>[2x]MNIQSTIKAVAETISTGPIPGSRKVYQAGELFPELRVPFREVAVHPSANEPPVTIYDPSGPYSDPAIQIDIEKGLPRTREALVVARGDVEEVADPRQVKPEDNGFAQGKHLAPEFPDTGRKIYRAKPGKLVTQLEYARAGIITAEMEYVAIRENLRREQDRPCVRDGEDFGASIPDFVTPEFVRQEIARGRAIIPANINHGELEPMAIGRNFLVKINANIGNSAVLSTVADEVDKLVWATRWGADTVMDLSTGRNIHNIRDWIIRNSSVPIGTVPIYQALEKVNGVAEDLNWEVFRDTLIEQCEQGVDYFTIHAGVRLPFIPMTAKRVTGIVSRGGSIMAKWCLAHHKENFLYERFDEICEIMRAYDVSFSLGDGLRPGSTADANDEAQFSELRTLGELTKVAWKHGVQVMIEGPGHVAMHKIKANMDEQLKHCHEAPFYTLGP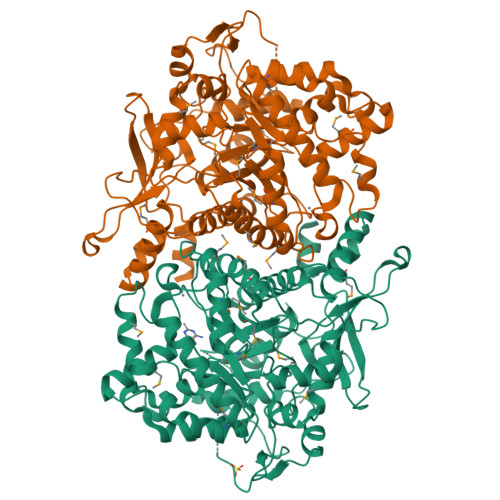LTTDIAPGYDHITSAIGAAMIGWFGTAMLCYVTPKEHLGLPDRDDVKTGVITYKLAAHAADLAKGHPGAAMWDDAISRARFEFRWEDQFNLGLDPETARKFHDETLPKEAHKTAHFCSMCGPKFCSMKISQEVRDFAAGKAPNSAELGMAEMSEKFREQGSEIYLKTE> DNRLGLV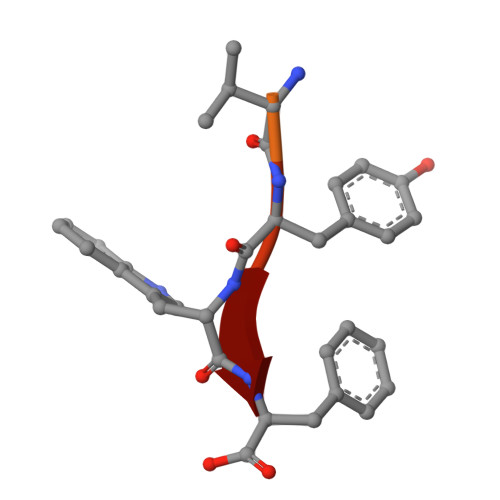YWF Here we report the biochemical characterization of the AA12 enzyme encoded by the genome of the ascomycete Trichoderma reesei (TrAA12). The three-dimensional structure of TrAA12 reveals important similarities with bacterial soluble glucose dehydrogenases (sGDH). TrAA12 preferentially oxidizes l-fucose, and weak activity was measured against d-arabinose (11.6% relative activity), d-galactose (5.7%), l-arabinose (2.8%), and d-lyxose (2.2%). Based on these results, the AA12 family of enzymes is likely to have a catalytic mechanism close to that of bacterial sGDH.

Soaking experiments were performed on native crystals in crystallization buffer supplemented with calcium, PQQ, and l-fucose. A large additional electron density inside a pocket and a reorganization of the amino acids surrounding this electron density were observed in each of the eight structures. Based on the difference map peak intensity, a part of the additional electron density was assigned to a second calcium ion. The calcium is directly coordinated by the side chain of Asp242 and the carbonyl of the Ser240 and is completed by two water molecules. A third water molecule completes this well-organized network. This organization is conserved in the native crystal, where the calcium ion is replaced by a water molecule. The superimposition of the catalytic calcium structure with the native one shows a movement of the loop spanning residues Thr353 to Thr357. Asp354 presents the largest difference, with a displacement of 1.55 Å of its C-α and a change of the orientation of its side chain. The new side chain position of Asp354 is stabilized by two new hydrogen bonds with Asp243. These movements partially close a part of the binding site and bring the side chains of Asp242 and Thr353 near the putative substrate binding site.

> CTTNNLQVTYPAPVAADGWEYRLISTGLTAPRSIVFDSTGGLLVLDAGVGVRRLTLQDNGGTCLSVTANATLIADTALNHGLAISADGGTIYASTVNDVYAYTYNEQTNTVDPTTRRTVVTNMTNTDHVTRTLLLSSRLPNELLVSRGSAANEDPQARNVTSGHSQIRAYDISTLAATDPPFDFVAGTLIGWGLRDSVGVGENPTNGGIWSVENSVDDLTREGVDVHQDNPGEELNFHGILGNTANQGGNYGYPDCYALWSTAGFPDLGALEVGDQFASDNATAGVTDATCNTNFVDPRLVFQAHVSPLDIKFNTNGTTAYITFHGSTDRTTPVGYSIVSVAFGLNGQPTSPMDSTTAANNILTSPDLTQCPDDCFTPVGLTFDTIGRLFFSSDSTGEIFVLQQS> GPLGSMWERLNCAAEDFYSRLLQKFNEEKKGIRKDPFLYEADVQVQLISKGQPNPLKNILNENDIVFIVEKVPLEKEETSHIEELQSEETAISDFSTGENVGPLALPVGKARQLIGLYTMAHNPNMTHLKINLPVTAL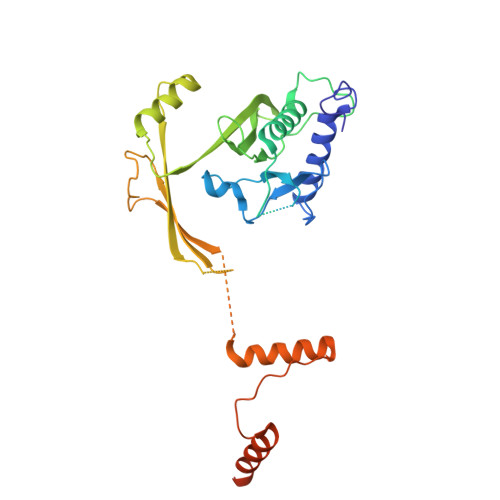PPLWVRCDSSDPEGTCWLGAELITTNNSITGIVLYVVSCKADKNYSVNLENLKNLHKKRHHLSTVTSKGFAQYELFKSSALDDTITASQTAIALDISWSPVDEILQIPPLSSTATLNIKVESGEPRGPLNHLYRELKFLLVLADGLRTGVTEWLEPLEAKSAVELVQEFLNDLNKLDGFGDSTKKDTEVETLKHDTAAVDR(3-NITRO-5-(3-MORPHOLIN-4-YL-PROPYLAMINOCARBONYL)PHENYL)-GALACTOPYRANOSIDE 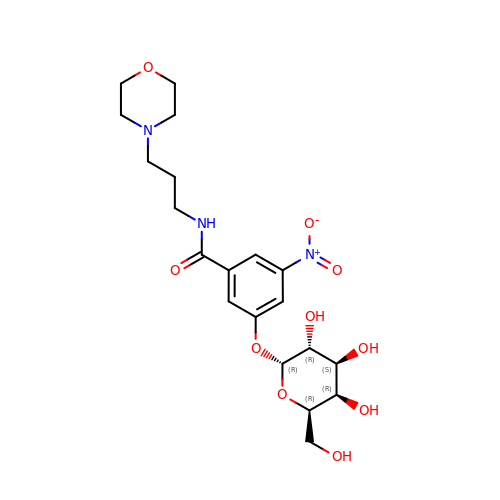| C20 H29 N3 O10 | CBPMHEKCQNCVNT-QTVCLEQKSA-N>[4x]REWFLHRNSLIVLADVALFLALYHFLPFEHNVVLGISMLAFIAVLWLTEALHVTVTAILVPVMAVFFGIFETQAALNNFANSIIFLFLGGFALAAAMHHQGLDKVIADKVLAMAQGKMSVAVFMLFGVTALLSMWISNTATAAMMLPLVLGVLSKVDADKQRSTYVFVLLGVAYSASIGGIATLVGSPPNAIAAAEVG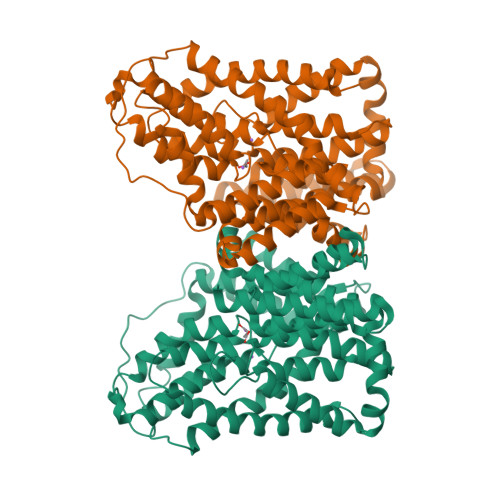LSFTDWMKFGLPTAMMMLPMAIAILYFLLKPTLNGMFELDRAPVNWDKGKVVTLGIFGLTVFLWIFSSPINAALGGFKSFDTLVALGAILMLSFARVVHWKEIQKTADWGVLLLFGGGLCLSNVLKQTGTSVFLANALSDMVSHMGIFVVILVVATFVVFLTEFASNTASAALLIPVFATVAEAFGMSPVLLSVLIAVAASCAFMLPVATPPNAIVFASGHIKQSEMMRVGLYLNIACIGLLTAIAMLFWQ> MDKKTIYFICTGNSARSQMAEGWGKEILGEGWNVYSAGIETHGVNPKA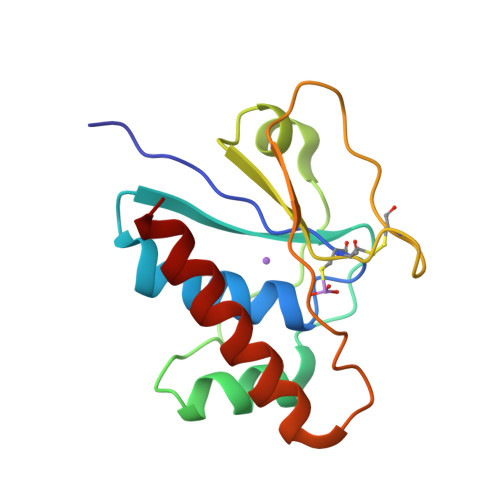IEAMKEVDIDISNHTSDLIDNDILKQSDLVVTLCSDADNNCPILPPNVKKEHWGFDDPAGKEWSEFQRVRDEIKLAIEKFKLR>[4x]SNAMARILKTAYTFDDVLLVPNKSEVLPNEVSLKTQLTKKIQLNIPLMSASMDTVTESKMAIAMAREGGIGIIHKNMTIEDQAREVDRVKRSGGLLCGASIGVTNDMMERVDAVVKAKVDVIVLDTAHGHSKGVIEGVKRIKAKYPELQVIAGNIATPE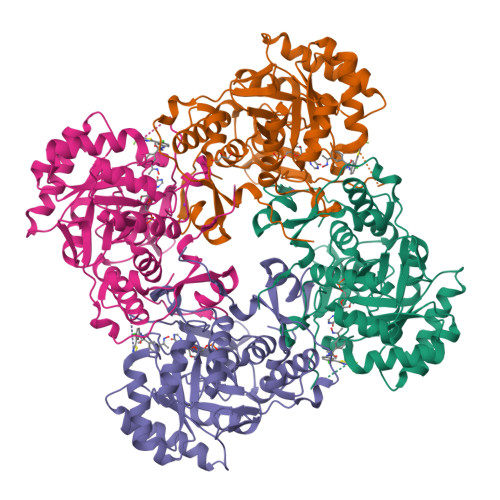AVRDLAEAGADCVKVGIGPGSICTTRIVAGVGVPQLTAVMDCAEEGKKLGIPVIADGGLKYSGDIVKALAAGACAAMMGSIFAGCEEAPGAIEIYQGRSYKVYRGMGSLGAMAKGSSDRYFQNGTKKFVPEGVEGRIAYKGHLADTIYQLIGGIKSGMGYLGAPTLENLYENANFVVQTSAGFRESHPHDINITKEAPNYSVNQ The Escherichia coli enzyme EcAIII catalyzes the hydrolysis of L‐Asn to L‐Asp and ammonia. Using a nature‐inspired mutagenesis approach, we designed and produced five new EcAIII variants (M200I, M200L, M200K, M200T, M200W). The modified proteins were characterized by spectroscopic and crystallographic methods. All new variants were enzymatically active, confirming that the applied mutagenesis procedure has been successful.

The determined crystal structures revealed new conformational states of the EcAIII molecule carrying the M200W mutation and allowed a high‐resolution observation of an acyl‐enzyme intermediate with the M200L mutant.

>[2x]MGKAVIAIHGGAGAISRAQMSLQQELRYIEALSAIVETGQKMLEAGESALDVVTEAVRLLEECPLFNAGIGAVFTRDETHELDACVMDGNTLKAGAVAGVSHLRNPVLAARLVMEQSPHVMMIGEGAENFAFARGMERVSPEIFSTSLRYEQLLAARKEGATVLDHSGAPLDEKQKMG;> TVGAVALDLDGNLAAATSTGGLTNKLPGRVGDSPLVGAGCYANNASVAVSCTGTGEVFIRALAAYDIAALMDYGGLSLAEACERVVMEKLPALGGSGGLIAIDHEGNVALPFNTEGMYRAWGYAGDTPTTGIYREKGDTVATQ;> DVGAVALDLDGNLAAATSTGGLTNKLPGRVGDSPLVGAGCYANNASVAVSCTGTGEVFIRALAAYDIAALMDYGGLSLAEACERVVMEKLPALGGSGGLIAIDHEGNVALPFNTEGMYRAWGYAGDTPTTGIYREKGDTVATQ The RNA-targeting type III-E CRISPR-gRAMP effector interacts with a caspase-like protease TPR-CHAT to form the CRISPR-guided caspase complex (Craspase), but their functional mechanism is unknown. Here, we report cryo-EM structures of the type III-E gRAMPcrRNA and gRAMPcrRNA-TPR-CHAT complexes, before and after either self or non-self RNA target binding, and elucidate the mechanisms underlying RNA-targeting and non-self RNA-induced protease activation. A recently characterized type III-E CRISPR-Cas subtype contains a single-protein effector that exhibits specific target RNA cleavage activity with no collateral activity or cell toxicity, representing a promising new tool for manipulating RNA. Lacking the type III signature protein Cas10, the III-E CRISPR loci often contain a gene encoding a caspase-like protease called TPR-CHAT that contains a caspase HetF associated with TPRs (CHAT) domain, which is a caspase family protease typically involved in programmed cell death, fused with a tetratricopeptide repeat (TPR) domain.

The nucleotides at positions −1 to −16 in the 18-nt 5′-repeat tag formed multiple sequence-specific contacts with residues in Csm4 and Csm3, indicating gRAMP recognizes the 5′-repeat tag in a sequence-dependent manner, consistent with the conservation of the 5′-repeat tag sequence. In contrast, we found a series of sequence-nonspecific contacts between the crRNA spacer sequence and Csm3.1, Csm3.2, and Csm5, accounting for the lack of sequence specificity for spacer sequence recognition. Notably, a metal ion was coordinated by the phosphate group of −11U, the side chain of D137, and the carboxyl group of G134 and A139 in the gRAMP complex (blue inset). A magnesium ion critical for guide RNA stabilization is located in a similar position in prokaryotic Argonautes29, suggesting the metal ion observed here may also function in stabilizing the 5′-repeat tag in the gRAMP complex. By contrast, in the type III-E gRAMPcrRNA complex, nucleotides −1C and −2A within the 5′-repeat tag stack with 1C to 3A within the spacer, which are available for base pairing with the self RNA target (red inset), possibly acting as sensors to discriminate self and non-self RNA. In addition, the two cleavable phosphates were stabilized by residues in the Csm2 domain (black and green insets). Notably, these residues undergo substantial conformational changes revealed by the structural comparison between the gRAMPcrRNA-target RNA ternary complex and the gRAMPcrRNA binary, whose structure we determined at 2.7 Å.

> MHHHHHHKSNDMNITVELTFFEPYRLVEWFDWDARKKSHSAMRGQAFAQWTWKGKGRTAGKSFITGTLVRSAVIKAVEELLSLNNGKWEGVPCCNGSFQTDESKGKKPSFLRKRHTLQWQANNKNICDKEEACPFCILLGRFDNAGKVHERNKDYDIHFSNFDLDHKQEKNDLRLVDIASGRILNRVDFDTGKAKDYFRTWEADYETYGTYTGRITLRNEHAKKLLLASLGFVDKLCGALCRIEVIKKSESPLPSDTKEQSYTKDDTVEVLSEDHNDELRKQAEVIVEAFKQNDKLEKIRILADAIRTLRLHGEGVIEKDELPDGKEERDKGHHLWDIKVQGTALRTKLKELWQSNKDIGWRKFTEMLGSNLYLIYKKETGGVSTRFRILGDTEYYSKAHDSEGSDLFIPVTPPEGIETKEWIIVGRLKAATPFYFGVQQPSDSIPGKEKKSEDSLVINEHTSFNILLDKENRYRIPRSALRGALRRDLRTAFGSGCNVSLGGQILCNCKVCIEMRRITLKDSVSDFSEPPEIRYRIAKNPGTATVEDGSLFDIEVGPEGLTFPFVLRYRGHKFPEQLSSVIRYWEENDGKNGMAWLGGLDSTGKGRFALKDIKIFEWDLNQKINEYIKERGMRGKEKELLEMGESSLPDGLIPYKFFEERECLFPYKENLKPQWSEVQYTIEVGSPLLTADTISALTEPGNRDAIAYKKRVYNDGNNAIEPEPRFAVKSETHRGIFRTAVGRRTGDLGKEDHEDCTCDMCIIFGNEHESSKIRFEDLELINGNEFEKLEKHIDHVAIDRFTGGALDKAKFDTYPLAGSPKKPLKLKGRFWIKKGFSGDHKLLITTALSDIRDGLYPLGSKGGVGYGWVAGISIDDNVPDDFKEMINKTEMPLPEEVEESNNGPINNDYVHPGHQSPKQDHKNKNIYYPHYFLDSGSKVYREKDIITHEEFTEELLSGKINCKLETLTPLIIPDTSDENGLKLQGNKPGHKNYKFFNINGELMIPGSELRGMLRTHFEALTKSCFAIFGEDSTLSWRMNADEKDYKIDSNSIRKMESQRNPKYRIPDELQKELRNSGNGLFNRLYTSERRFWSDVSNKFENSIDYKREILRCAGRPKNYKGGIIRQRKDSLMAEELKVHRLPLYDNFDIPDSAYKANDHCRKSATCSTSRGCRERFTCGIKVRDKNRVFLNAANNNRQYLNNIKKSNHDLYLQYLKGEKKIRFNSKVITGSERSPIDVIAELNERGRQTGFIKLSGLNNSNKSQGNTGTTFNSGWDRFELNILLDDLETRPSKSDYPRPRLLFTKDQYEYNITKRCERVFEIDKGNKTGYPVDDQIKKNYEDILDSYDGIKDQEVAERFDTFTRGSKLKVGDLVYFHIDGDNKIDSLIPVRISRKCASKTLGGKLDKALHPCTGLSDGLCPGCHLFGTTDYKGRVKFGFAKYENGPEWLITRGNNPERSLTLGVLESPRPAFSIPDDESEIPGRKFYLHHNGWRIIRQKQLEIRETVQPERNVTTEVMDKGNVFSFDVRFENLREWELGLLLQSLDPGKNIAHKLGKGKPYGFGSVKIKIDSLHTFKINSNNDKIKRVPQSDIREYINKGYQKLIEWSGNNSIQKGNVLPQWHVIPHIDKLYKLLWVPFLNDSKLEPDVRYPVLNEESKGYIEGSDYTYKKLGDKDNLPYKTRVKGLTTPWSPWNPFQVIAEHEEQEVNVTGSRPSVTDKIERDGKMV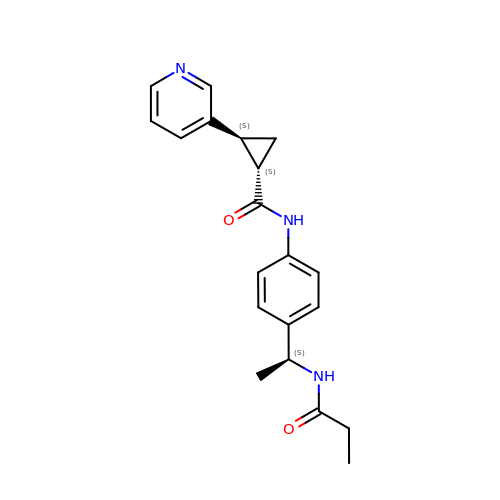(1S,2S)-N-{4-[(1S)-1-(propanoylamino)ethyl]phenyl}-2-(pyridin-3-yl)cyclopropane-1-carboxamide | C20 H23 N3 O2 | KBYVLVXBCRUYTD-VHSSKADRSA-N>[2x]G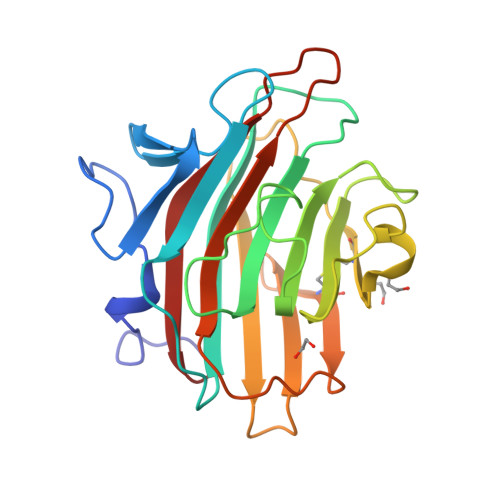SDASKLSSDYSLPDLINTRKVPNNWQTGEQASLEEGRIVLTSNQNSKGSLWLKQGFDLKDSFTMEWTFRSVGYSGQTDGGISFWFVQDSNIPRDKQLYNGPVNYDGLQLLVDNNGPLGPTLRGQLNDGQKPVDKTKIYDQSFASCLMGYQDSSVPSTIRVTYDLEDDNLLKVQVDNKVCFQTRKVRFPSGSYRIGVTAQNGAVNNNAESFEIFKMQFFNGV> GSMADEATRRVVSEIPVLKTNAGPRDRELWVQRLKEEYQSLIRYVENNKNADNDWFRLESNKEGTRWFGKCWYIHDLLKYEFDIEFDIP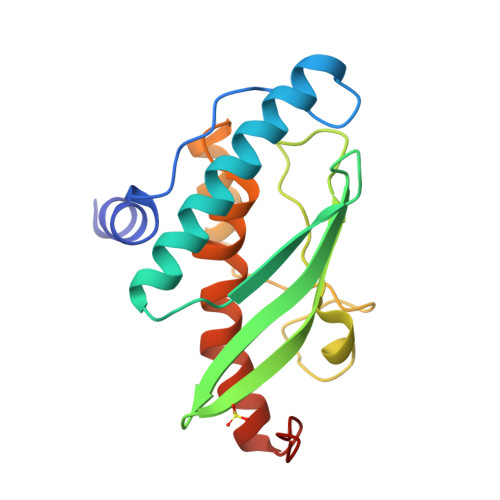ITYPTTAPEIAVPELDGKSAKMYRGGKICLTDHFKPLWARNVPKFGLAHLMALGLGPWLAVEIPDLIQKGVIHHKEKCNQ>[2x]MIPARFAGVLLALALILPGTLCAEGTRGRSSTARCSLFGSDFVNTFDGSMYSFAGYCSYLLAGGCQKRSFSIIGDFQNGKRVSLSVYLGEFFDIHLFVNGTVTQGDQRVSMPYASKGLYLETEAGYYKLSGEAYGFVARIDGSGNFQVLLSDRYFNKTCGLCGNFNIFAEDDFMTQEGTLTSDPYDFANSWALSSGEQWCERASPPSSSCNISSGEMQKGLWEQCQLLKSTSVFARCHPLVDPEPFVALCEKTLCECAGGLECACPALLEYARTCAQEGMVLYGWTDHSACSPVCPAGMEYRQCVSPCARTCQSLHINEMCQERCVDGCSCPEGQLLDEGLCVESTECPCVHSGKRYPPGTSLSRDCNTCICRNSQWICSNEECPGECLVTGQSHFKSFDNRYFTFSGICQYLLARDCQDHSFSIVIETVQCADDRDAVCTRSVTVRLPGLHNSLVKLKHGAGVAMDGQDVQLPLLKGDLRIQHTVTASVRLSYGEDLQMDWDGRGRLLVKLSPVYAGKTCGLCGNYNGNQGDDFLTPSGLAEPRVEDFGNAWKLHGDCQDLQKQHSDPCALNPRMTRFSEEACAVLTSPTFEACHRAVSPLPYLRNCRYDVCSCSDGRECLCGALASYAAACAGRGVRVAWREPGRCELNCPKGQVYLQCGTPCNLTCRSLSYPDEECNEACLEGCFCPPGLYMDERGDCVPKAQCPCYYDGEIFQPEDIFSDHHTMCYCEDGFMHCTMSGVPGSLLPDAVLSSPLSHRSKRSLSCRPPMVKLVCPADNLRAEGLECTKTCQNYDLECMSMGCVSGCLCPPGMVRHENRCVALERCPCFHQGKEYAPGETVKIGCNTCVCRDRKWNCTDHVCD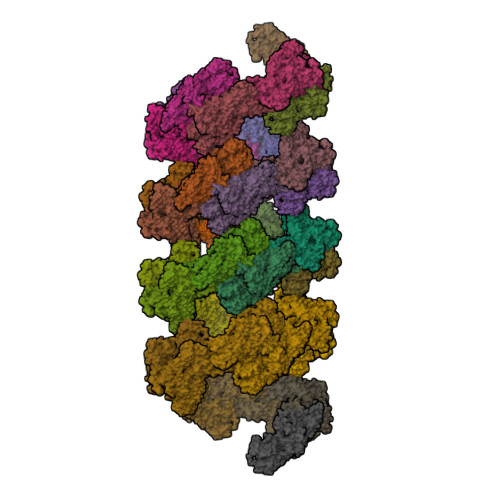ATCSTIGMAHYLTFDGLKYLFPGECQYVLVQDYCGSNPGTFRILVGNKGCSHPSVKCKKRVTILVEGGEIELFDGEVNVKRPMKDETHFEVVESGRYIILLLGKALSVVWDRHLSISVVLKQTYQEKVCGLCGNFDGIQNNDLTSSNLQVEEDPVDFGNSWKVSSQCADTRKVPLDSSPATCHNNIMKQTMVDSSCRILTSDVFQDCNKLVDPEPYLDVCIYDTCSCESIGDCACFCDTIAAYAHVCAQHGKVVTWRTATLCPQSCEERNLRENGYECEWRYNSCAPACQVTCQHPEPLACPVQCVEGCHAHCPPGKILDELLQTCVDPEDCPVCEVAGRRFASGKKVTLNPSDPEHCQICHCDVVNLTCEACQEPGHHHHHH(3~{R})-~{N}-[3-(3,4-dihydro-2~{H}-quinolin-1-yl)-2,2-bis(fluoranyl)propyl]-3-methyl-2-oxidanylidene-3,4-dihydro-1~{H}-quinoxaline-5-carboxamide 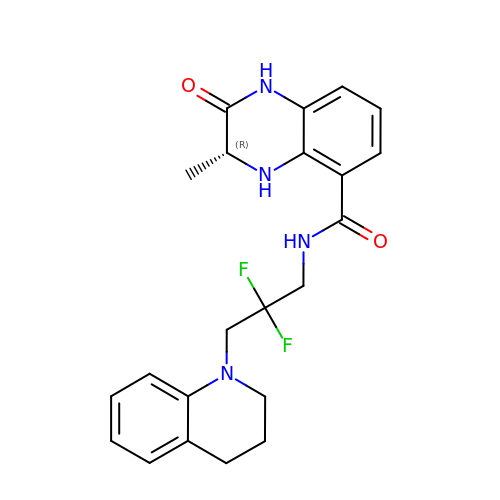| C22 H24 F2 N4 O2 | HTEQIZSWLJNYLH-CQSZACIVSA-N>MKAYMFPGQGSQAKGMGRALFDAFPALTARADGVLGYSIRALCQDDPDQRLSQTQFTQPALYVVNALSYLKRREEEAPPDFLAGHSLGEFSALFAAGVFDFETGLALVKKRGELMGDARGGGMAAVIGLDEERVRELLDQNGATAVDIANLNSPSQVVISGAKDEIARLQVPFEAAGAKKYTVLRVSAAFHSRFMRPAMVEFGRFLEGYDFAPPKIPVISNVTARPCKADGIRAALSEQIASPVRWCESIRYLMGR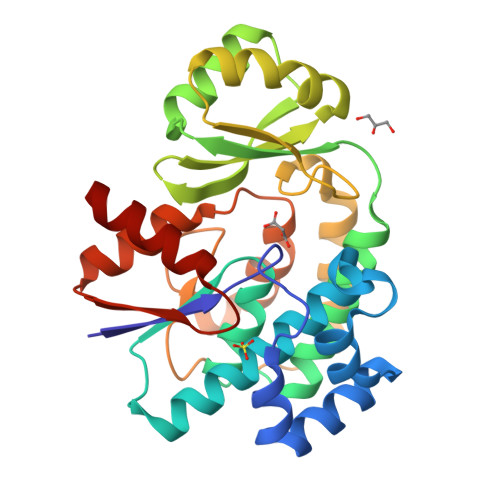GVEEFVECGHGIVLTGLYAQIRRDA[2x]Borussertib | C36 H34 N6 O3 | 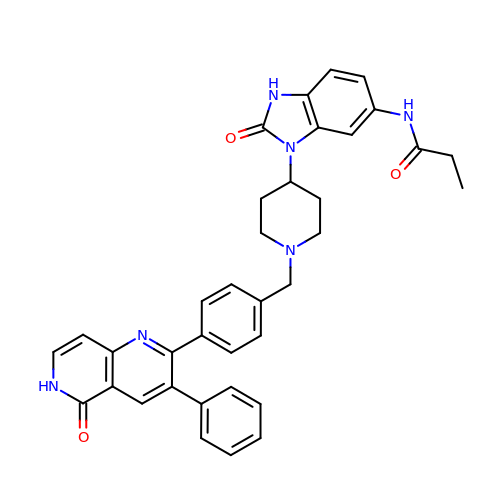NFXSQFADJLOQHR-UHFFFAOYSA-N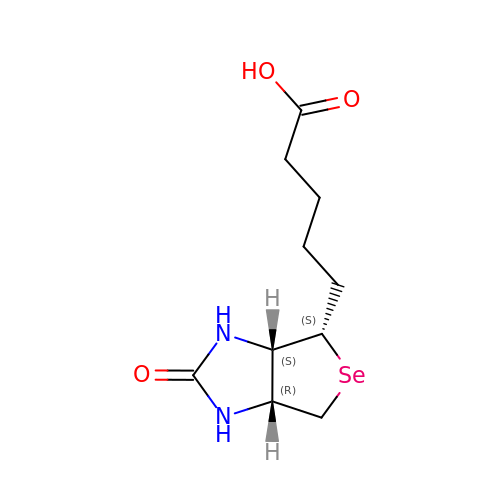5-[(3aS,4S,6aR)-2-oxohexahydro-1H-selenopheno[3,4-d]imidazol-4-yl]pentanoic acid | C10 H16 N2 O3 Se | HVUDXAKXEONARI-ZKWXMUAHSA-N>[6x]MEITSDMEEDKDLMLKLLDKNGFVLKKVEIYRSNYLAILEKRTNGIR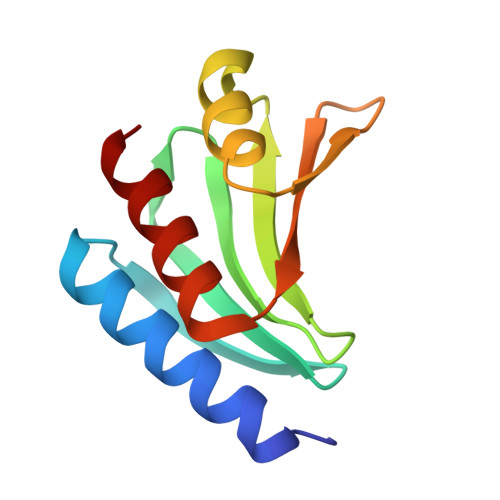NFEINNNGNMRIFGYKMMEHHIQKFTDIGMSCKIAKNGNVYLDIKRSAENIEAVITVASEL>GAMGSMATRIAILGAGPSGMAQLRAFQSAQEKGAEIPELVCFEKQADWGGQWNYTWRTGLDENGEPVHSSMYRYLWSKGPKECLEFADYTFDEHFGKPIASYPPREVLWDYIKGRVEKAGVRKYIRFNTAVRHVEFNEDSQTFTVTVQDHTTDTIYSAAFDYVVCCTGHFSTPYVPEFEGFEKFGGRILHAHDFRDALEFKDKTVLLVGSSYSAEDIGSQCYKYGAKKLISCYRTAPMGYKWPENWDERPNLVRVDTENAYFA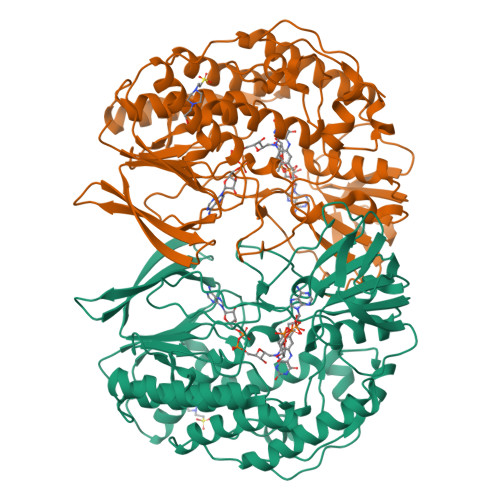DGSSEKVDAIILCTGYIHHFPFLNDDLRLVTNNRLWPLNLYKGVVWEDNPKFFYIGMQDQWYSFNMFDAQAWYARDVIMGRLPLPSKEEMKADSMAWREKELTLVTAEEMYTYQGDYIQNLIDMTDYPSFDIPATNKTFLEWKHHKKENIMTFRDHSYRSLMTGTMAPKHHTPWIDALDDSLEAYLSDKSEIPVAKEA[4x]>IHPKNRWYKAWEMFILVWAIYSSLFTPMEFGFFRGLPERLFVLDIVGQIAFLVDIVLQFFVAYRDTQTYRTVYKPTRIAFRYLKSHFLMDFIGCFPWDLIYKASGKHELVRYLLWIRLFRVRKVVEFFQRLEKDTRINYLFTRILKLLFVEVYCTHTAACIFYYLATTLPPENEGYTWIGSLKLGDYSYENFREIDLWKRYTTALYFAIVTMATVGYGDIHAVNLREMIFVMIYVSFDMVLGAYLIGNITALIVKG[4x]

GORK is a shaker-like potassium channel in plants that contains ankyrin (ANK) repeats. GORK, also known as guard cell outward rectifying K+ channel, is the only outward-rectifying potassium channel in guard cells. In contrast, GORK activation causes potassium efflux, reducing guard cell turgor and volume and in turn stomatal closure. Each protomer has an N-terminal transmembrane domain (TMD, residues 58–313, containing helices S1–S6), followed by three cytoplasmic domains: the C-linker (residues 314–365), cyclic nucleotide-binding domain homolog (CNBDH) (residues 366–510), and ANK (residues 511–724).

We determined the cryo-EM structures of the full-length AtGORK (AtGORKFL, residues 1–820) in an autoinhibited state, along with two ANK-truncated versions (AtGORK623, residues 1–623; AtGORK510, residues 1–510). For the truncated AtGORK510 and AtGORK623, cryo-EM maps at 3.4 Å and 3.2 Å resolution, respectively, were obtained. Both maps showed high-quality density in their transmembrane domain, allowing accurate modeling, while the flexible cytosolic domains remained unmodeled due to their invisibility. Removing the KHA domain while retaining the intact ANK domain in AtGORK (Δ737–820, residues 1–736) led to a slight increase in oocytes currents, whereas deleting the last three C-terminal ANK repeats (Δ624–820, residues 1–623) significantly enhanced current amplitude—reaching 13.3-fold that of the full-length channel at +70 mV. Structural reconstructions of AtGORK623 and AtGORK510 resolved only the TMD portion, with their cytoplasmic regions remaining unresolved due to their intrinsic flexibility. While the absence of density in these regions limits direct visualization of cytoplasmic symmetry, it likely reflects increased structural mobility upon ANK truncation, supporting the conclusion that ANK removal disrupts autoinhibitory interactions and converts GORK into an activatable state. Firstly, the structures of AtGORK623 and AtGORK510 are highly similar, with a root-mean-square deviation (RMSD) of approximately 0.48 Å for their superimposed tetramers. Importantly, the ANK-truncated protomers exhibit strict C4 symmetry, with RMSDs of approximately 0.16 Å/256 superimposed Cα. A comparison of protomers A and B in both AtGORKFL1 and AtGORK623 reveals that the protomers in AtGORK623 closely resemble protomer A in AtGORKFL1, rather than protomer B. This suggests that ANK dimerization results in C2 symmetry in the full-length AtGORKFL1, whereas ANK truncation restores C4 symmetry in the AtGORK623.>ETLVRPKPLLLKLLKSVGAQKDTYTMKEVLFYLGQYIMTKRLYDEKQQHIVYCSNDLLGDLFGVP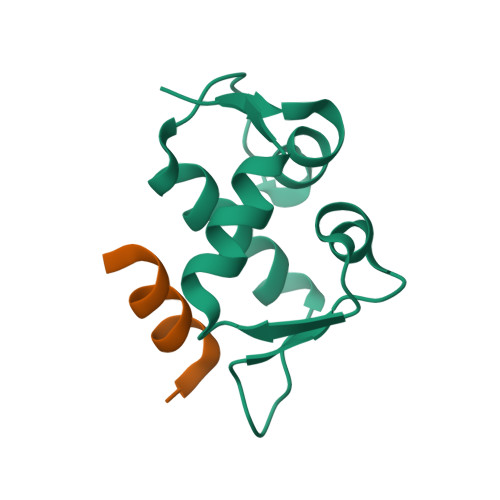SFSVKEHRKIYTMIYRNLVV[2x];>[2x]LTFLEYWAQLMQ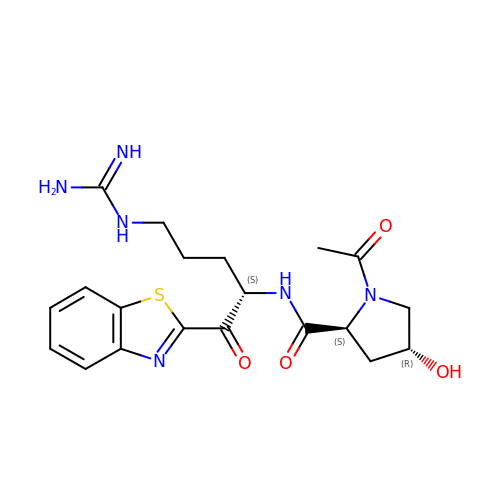(2S,4R)-1-ACETYL-N-[(1S)-4-[(AMINOIMINOMETHYL)AMINO]-1-(2-BENZOTHIAZOLYLCARBONYL)BUTYL]-4-HYDROXY-2-PYRROLIDINECARBOXAMIDE | C20 H26 N6 O4 S | VXDAVYUFYPFGDX-SNPRPXQTSA-N> SSGKMNEWESLNTTLNRFTDNVVKFRRDSRTKALKCWRPIVDGIVDYVKRKDDRFHALSVFHKGSYYERSKVGEPDEFDLMLVMDNLELYDEPFEEDDGLSEPPIGFTTVMIDQGEEKPWKRDECVNRRGMLNATRVKAVFKRLADEAIQDMKSKGHWRNVTVKSGGTAV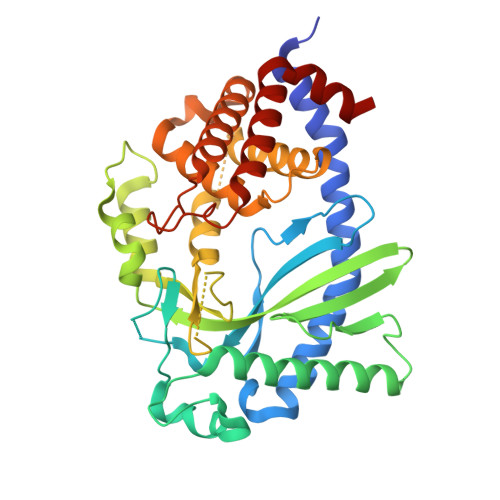TLKISKDGREYSVDLTLGIKDNTWPEDAEEWKTRQRKGWPKRNLVHDIHEMGCHLVTKQPKGHSPIEQERGFLWCYSFSEAEKKLFLQGEQGEVNSCRRQVLRILKALREELELQPLKSYHLKTLLLYECESQPSARQWSKDALSERFLDLLKRLEKCLRSKECPHYFIKDLNLFEMLNPEKCDELADRVNKILKQPGQVLIRLIK Integrin-linked kinase (ILK) is one of the few evolutionarily conserved proteins found in FAs to critically control the FA assembly and integrin–actin connection. However, sequence analysis suggested that despite containing kinase-like domain, ILK is a pseudokinase lacking several key active site residues. Our results reveal that by recruiting FA adaptors PINCH and Parvin into a heterotrimeric complex (IPP), ILK is able to trigger F-actin filament bundling via two WASP-Homology-2 actin-binding motifs, one from PINCH and the other from Parvin.

On the other hand, another major puzzle still remains unresolved, i.e., what is the role of Mg-ATP bound to the ILK pseudoactive site? To circumvent this problem, we carefully analyzed the ATP-binding residues in the pseudokinase domain of ILK structure and designed L207W mutation that does not affect the structural integrity but sterically occludes ATP binding to ILK. To validate our design, we first examined the propensity of the substitution by characterizing the recombinant ILK KLD L207W in complex with α-Parvin CH2. Consistently, CD denaturation studies revealed that there was little change in the thermal melting temperature of the mutant ILK (L207W) complex (Tm = 53.9 °C) versus that of the wild-type complex (Tm = 54.2 °C), demonstrating that the L207W substitution has little effect on the stability of ILK/Parvin complex. To further prove this, we solved the crystal structure of the ILK (L207W)/α-Parvin CH2 complex, which showed that the mutant complex exhibits the same interface as the WT complex, yet the substitution of L207 by more bulky side chain of tryptophan in the pseudokinase domain precluded the binding of ATP as well as Mg2+ as expected. The mutation clearly abolished the ATP binding as well as Mg2+ binding to ILK. We note here that Mg2+, while interacting with D339 at the pseudoactive site, is predominantly chelated to ATP 13,14 explaining why the loss of ATP binding also led to the loss of Mg2+ binding. Next, we examined the ability of IPP L207W mutant in affecting the F-actin bundle formation. Strikingly, as compared with WT IPP, loss of Mg-ATP in IPP L207W led to dramatically impaired F-actin bundling (Fig. 6b vs. 6c) with notable decrease in size of the formed F-actin bundles. Consequently, the mutation further reduced cell spreading and migration. It is important to note that like WT IPP, IPP L207W binds potently to F-actin. Another major finding of this study was that the IPP WH2-mediated F-actin bundling is highly sensitized to Mg-ATP bound to the pseudoactive site of ILK.

> MNKHSGIDFKQLNFLTKLNENHSGEWWKGRWQGNDIVVKVLKVRDWSTRKSRDFNEECPRLRIFSHPNVLPVLGACQSPPAPHPTLITHWMPYGSLYNVLHEGTNFVVDQSQAVKFALDMARGMAFLHTLEPLIPRHALNSRSVMIDEDMTARISMADVKFSFQSPGRMYAPAWVAPEALQKKPEDTNRRSADMWSFAVLLWELVTREVPFADLSNMEIGMKVALEGLRPTIPPGISPHVSKLMKICMNEDPAKRPKFDMIVPILEKMQDK;> GSHMDAFDTLFDHAPDKLNVVKKTLITFVNKHLNKLNLEVTELETQFADGVYLVLLMGLLEGYFVPLHSFFLTPDSFEQKVLNVSFAFELMQDGGLEKPKPRPEDIVNCDLKSTLRVLYNLFTKYRNVE5-[7-(difluoromethyl)-6-(1-methyl-1H-pyrazol-4-yl)-3,4-dihydroquinolin-1(2H)-yl]-3-methyl-1,3-benzothiazol-2(3H)-one 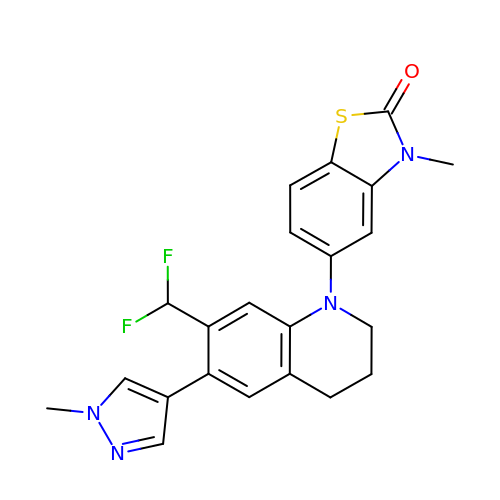| C22 H20 F2 N4 O S | WJHMCLBLUFFBIF-UHFFFAOYSA-N>GSHMQQVNPDFIEALTEKITEEVTAKVTEELTKQNMEFFAAVAKQSQDNFDRINKRLEERDEKLMSTIRLIQEQKSANAQ[4x]

Type I and II partition systems employ a Walker-type ATPase ParA and an actin-like ATPase ParM, respectively, whereas type III systems use an FtsZ/tubulin-like GTPase TubZ. TubY is a DNA-binding protein with a putative helix-turn-helix (HTH) motif that functions as a transcriptional activator of the tubRZ operon. More importantly, TubY modulates the interaction between the segrosome and the TubZ filaments; however, it remains unclear how TubY is involved in plasmid segregation. TubY, a putative MerR family protein, is considered to be an integral element of plasmid partitioning in type III par systems. This study shows that B. cereus TubY is a novel membrane-binding transcription factor and segrosome component by binding to the TubR-centromere complex, suggesting that the cell membrane is involved in the process of type III systems.

Here, I report the crystal structure of the TubY C-terminal coiled-coil domain of the pXO1-like plasmid pBc10987 from Bacillus cereus. Sequence analyses revealed that BcYN and BcYCΔ contain the HTH motif and coiled-coil domains, respectively. I determined the crystal structure of BcYCΔ. The asymmetric unit contains four BcYCΔ monomers, which forms a tetrameric four-helix bundle with dimensions 90 Å × 20 Å × 20 Å. These four monomers are parallel and related by a pseudo-2-fold axis, and the root-mean-square deviation (rmsd) of Cα atoms (residues 112–174 of chain A and B versus C and D) is 0.37 Å. The BcYCΔ structure reveals that the hydrophobic core of the four-helix bundle is mostly aliphatic. Regarding BcY, BcYN is monomeric and incapable of binding to DNA, whereas BcYC is a tetrameric parallel coiled-coil with no cysteine or histidine residues. The crystal structure of the BcY C terminus revealed that the coiled-coil region is a parallel tetramerization domain, demonstrating that BcY is a unique tetrameric MerR-like transcriptional regulator. The results of this study show that oligomerization enables efficient binding of BcY to DNA. GFP-BcYtail was not localized to the cell periphery, indicating that a single BcYtail peptide is not sufficient for the membrane attachment, and that tetramerization by the BcYCΔ region increases the affinity of BcYtail for lipid membranes.Cyclohexanone monooxygenase (CHMO; EC 1.14.13.22) is an FAD‐ and NADPH‐dependent Baeyer–Villiger monooxygenase (BVMO). A wide variety of ketones are converted by CHMO into esters or lactones through the insertion of an oxygen atom on one side or the other of the carbonyl group. Among the retrieved sequences, a putative CHMO from Thermocrispum municipale DSM 44069 was found (TmCHMO; NCBI RefSeq: WP_028849141.1). While AcCHMO essentially lost its activity after 25 min incubation in 14 % acetonitrile at 20 °C, TmCHMO remained highly active (>80 %) for at least 20 h under these conditions. These thermostability and solvent‐tolerance data clearly show that TmCHMO is a substantially more robust biocatalyst than AcCHMO.

For a more in‐depth understanding of TmCHMO properties, its crystal structure in complex with FAD and NADP+ in the oxidized and reduced states were solved to a resolution of 1.22 and 1.60 Å. The overall structures of the oxidized and reduced forms share an almost identical conformation, with a root mean square deviation of 0.20 Å for the backbone Cα atoms. However, inspection of the active sites shows distinct alterations. In the reduced enzyme, the electron density corresponding to the nicotinamide moiety of NADP+ is disordered, with no well‐defined electron density. Furthermore, R329 of the oxidized enzyme is engaged in H‐bonds with the carboxamide group of NADP+ and the side chain of D59. Upon enzyme reduction, R329 moves away from NADP+ and points toward the isoalloxazine moiety of the flavin ring, which favors an electrostatic interaction between the positively charged guanidinium group of R329 and the negatively charged reduced flavin. Upon formation of the flavin peroxide and concomitant loss of the negative charge on the flavin ring, R329 would shift back to the conformation interacting with the NADP+, thereby making the catalytic center accessible to a ketone substrate.23d These results confirm that the formation of the negatively charged reduced flavin is associated with a localized rearrangement of the central elements of the catalytic site.

> MSTTQTPDLDAIVIGAGFGGIYMLHKLRNDLGLSVRVFEKGGGVGGTWYWNKYPGAKSDTEGFVYRYSFDKELLREYDWTTRYLDQPDVLAYLEHVVERYDLARDIQLNTEVTDAIFDEETELWRVTTAGGETLTARFLVTALGLLSRSNIPDIPGRDSFAGRLVHTNAWPEDLDITGKRVGVIGTGSTGTQFIVAAAKMAEQLTVFQRTPQYCVPSGNGPMDPDEVARIKQNFDSIWDQVRSSTVAFGFEESTVEAMSVSESERQRVFQQAWDKGNGFRFMFGTFCDIATNPEANAAAAAFIRSKIAEIVKDPETARKLTPTDLYAKRPLCNEGYYETYNRDNVSLVSLKETPIEEIVPQGVRTSDGVVHELDVLVFATGFDAVDGNYRAMNLRGRDGRHINEHWTEGPTSYLGVTKAGFPNMFMILGPNGPFTNLPPSIEAQVEWISDLIDKATREGLTTVEPTADAEREWTETCAEIANMTLFPKADSWIFGANIPGKRHAVMFYLGGLGNYRRQLADVADGGYRGFQLRGERAQAVA3-(4-BENZENESULFONYL-THIOPHENE-2-SULFONYLAMINO)-PHENYLBORONIC ACID | C16 H14 B N O6 S3 | 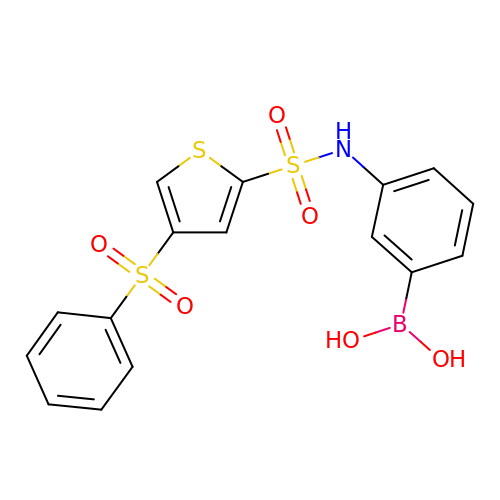YZOKHYPIQNIFRQ-UHFFFAOYSA-N>[4x]GPGKTDSSFIMDSDPRRCMRHHYVDSISHPLYKCSSKMVLLARCEGHCSQASRSEPLVSFSTVLKQPFRSSCHCCRPQTSKLKALRLRCSGGMRLTATYRYILSCHCEECNSGTETSQVAPA

Norrie Disease Protein (NDP) gene encodes Norrin, a secreted cystine-knot like growth factor, distinct from the lipid-modified Wnt. Unlike Wnts which have promiscuous interactions with Fz receptors, Norrin specifically binds to Fz4CRD, but not to the 14 other CRDs of Fz and secreted Frizzled-related protein (sFRP) family members. The Norrin mediated pathway maintains the blood-retina and blood-brain barriers and regulates angiogenesis in the cochlea and uterus as well as neuroprotective effects on retinal neurons. Our crystallographic and solution studies further reveal that dimeric Norrin forms a complex with two copies of monomeric Fz4CRD.

We determined three crystal structures of Norrin, using selenomethionine-labeled protein for phasing. The Norrin protein fold is identical to that of the previously reported MBP-Norrin crystal structure. Each Norrin monomer comprises three β-hairpins (β1-β2, β3-β4 and β5-β6), a β7 strand at the C-terminus, and four intramolecular disulphide bonds. The two monomers assemble as an elongated, head-to-tail, dimer stabilized by three intermolecular disulphide bridges (Cys93-Cys95, Cys95-Cys93, and Cys131-Cys131), in agreement with small-angle X-ray scattering (SAXS) measurements which showed Norrin dimer in solution. The dimer interface is further stabilized by extensive hydrogen bonds and hydrophobic interactions. Superposition of all molecules in the asymmetric units from our three crystal forms with the MBP-Norrin structure showed an average root-mean-square (r.m.s.) deviation of 1.5 Å over 190 equivalent Cα atoms. On inspection the superpositions revealed a high degree of conformational plasticity in the β1-β2, β3-β4 and β5-β6 loops. The flexibility inherent in these regions is consistent with the relatively high crystallographic B factor values. Conversely, the structural comparisons underscore the conserved nature of the interface at the dimer core.>MKVQYSFEREFEELMSDLLSKYGYEMFQMDGLGDQLDVVKFTEDFVRRGIIESTIDANANVRVTNISTYFIEISKPHTYLYSLYRIWQKMKEMFGKGVADEFVEAQINGAVYLHDRHHAALMPYCFAYTLKPIVEKGLPFIKTIKSEPAKHLSTFIQHVIQFVMFASNQSSGAVGLPDFFVWMWYFVKKDLKEGIIPRDKLDWYIEQHFQILTYSLNQPIRTTQSPYTNFTYLDRNYIKAIFEGERYPDGSLITDHVEDIIALQKHYWEWVSRERERQMFTFPVLTASLLYKDGKFLDEDSARFINKINMKWQDTNWYISDSIDAVASCCRLTSSTQTLKKFSLSSEEEEKLKGRMNSIGGSDLNIGSFKVITVNLPRIALESGGDREKYLQILRHRVQLIKKALAAVREIIKERISEGLLPLYENGLMLLNRQYGTIGVTGVWESASIMGLTTEDIDGLKYTEEGEVFVDNVLDTIREEAEKGYHEYGFTFNIEQVPAEKAAVTLAQKDRFLFGEKQPFEIYSNQWVPLMANTDVLNRIRYSGKWDKKVSGGAILHINLGESFKTEEESFNMVKMIADMGVMYFAFNTKISVCEDGHAFYGERCPVCGKAKVDEYMRIVGYLVPVSAFNKERREIEYPRRQFYDSLTIRR[2x]

Ribonucleotide reductases (RNRs) are highly important enzymes for all life, as they are solely responsible for the first committed step in the synthesis of the deoxyribonucleoside triphosphate (dNTP) building blocks of DNA. Class III RNRs, strictly anaerobic, generate on a separate activating enzyme NrdG the same type of 5’-dAdo radical through homolytic cleavage of a C-S bond in S-adenosylmethionine, with the participation of a [4Fe-4S] cluster. Here we present the crystal structure of a second class III RNR from Thermotoga maritima (tmNrdD), which, as purified and crystallized, surprisingly does not display such a cysteine, possessing an isoleucine (Ile) in its place. Nevertheless tmNrdD binds a substrate and its allosteric effector in productive conformations as expected from previous structures of RNRs of all three classes, and it is enzymatically active.

The structure of tmNrdD has also been determined in complex with the allosteric substrate specificity effector dATP and its cognate substrate CTP, as well as with dATP alone. The dATP/CTP complex represents the first structure of an anaerobic, class III RNR with a substrate and the first of any RNR in complex with a triphosphate substrate. The electron density is very well defined for all parts of the CTP nucleotide. The cytosine base stacks imperfectly on top of Tyr227, equivalent to Phe194 in T4NrdD. Effector binding induces a conformation of the substrate-proximal side of loop 2 that projects the side chains of Arg221 and Gln224 towards the substrate base, thereby enhancing CTP binding through three H-bonds between these side chains and its base. As in the other classes, the α and β phosphate groups of the substrate are held in place by several H-bonding interactions to the N-terminus of a conserved α-helix (499–514). The γ-phosphate group interacts with the side chain hydroxyl group of Tyr112, His114 and the main chain amide group of Asp115. With the ribose positioned as described, Ile359 at the tip of the finger loop is positioned in between the radical-bearing residue Gly621 and the substrate; however it does not reveal an obvious pathway for transfer of the radical (see Discussion). Furthermore the crystal structure of the dATP/CTP complex shows that the SIGG motif is compatible with substrate binding.>[8x]ARGTNVGREC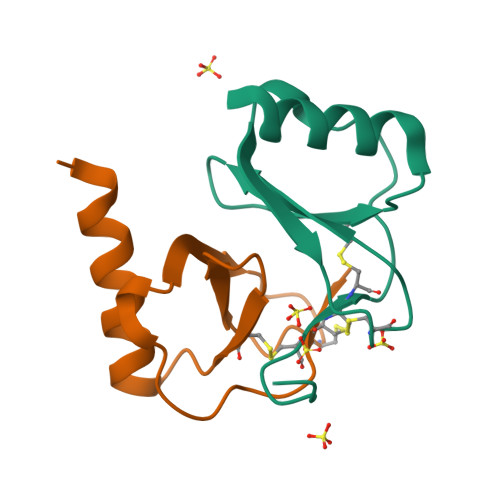CLEYFKGAIPLRKLKTWYQTSEDCSRDAIVFVTVQGRAICSDPNNKRVKNAVKYLQSLERS> SASIEKVNKLPKSPRNRFLLPPKGGTETTRRDIYNQILKDMAAFPENTIVTAVLASVDVTDNCAYVAKWDESSDRIKKVLQRQLPLQELDQLPDYGDIFAVLDSINNIITRITINSSSAGGGYDAYLIDFGEHIHFDGNETIFKLPDDIKRLPAQAIRCDLINCDIANMHCFVNTYIKIRVHENNNSTLVAEPVIDRLSRPTKTNTTKYPAGITEDDMAMLNEIDESTSDPLKAVLGF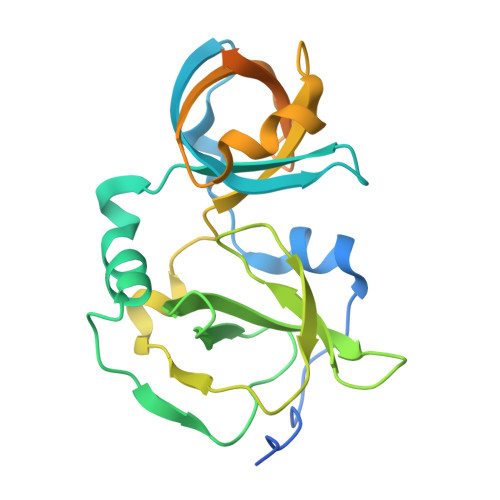RPKD2-chloro-N-(4-phenyl-1,3-thiazol-2-yl)benzamide 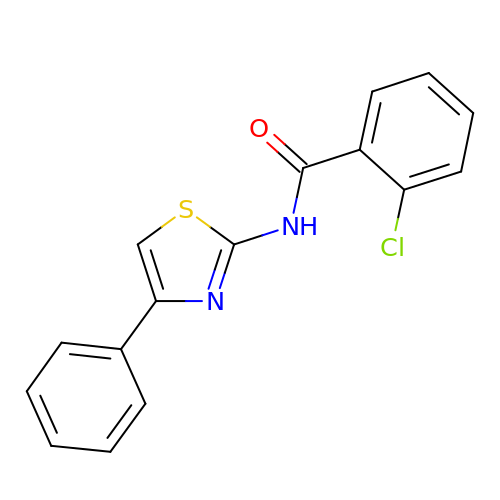| C16 H11 Cl N2 O S | FXJFKYBQUTVGOL-UHFFFAOYSA-N>GAINLYSSRHYDTDQALYDSFTKKTGLKVNLIEGKGDKLIERIKSEGANSPADVFMTVDAGRLWRAQEAGILQPISSSTLNNKIPANLRSPEKLWFGFSKRARVIMYNKNKVQPSELSTYEDLAQNKWKGKIVIRSSSNIYNQSLIA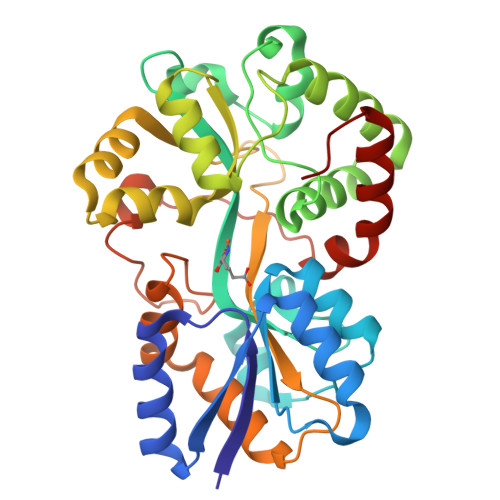SLIEIHGMSDAEGWAKGFVRNFARPPEGNDTAQIKAVAAGIGDIGLANSYYLARLKRSSKPEDQAVADKVGMFFPNQNGRGTHVNISGGGVVKNAPNKEGAIKFLEYLVSPEAQKIFSEGNNEYPVVAGVPIASVLKPFGSFKNDSTNVSVYGKLNADAIKLMDRVGWKLE[2x]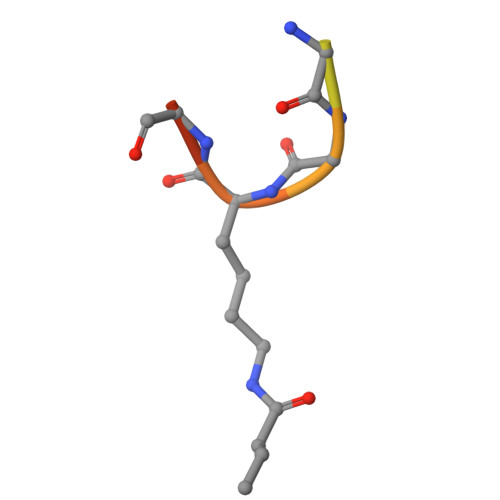> SGRGXGGXGLG>[2x]MCF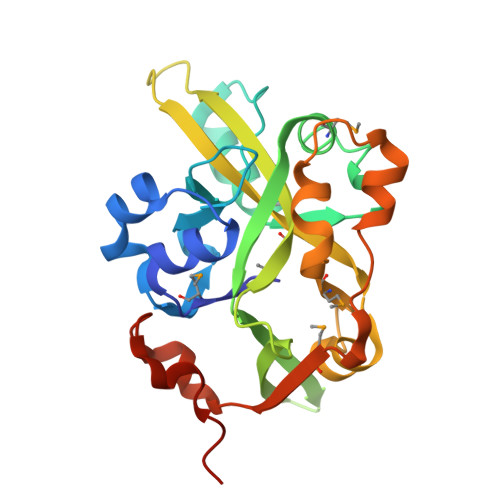HNSMSAKAIKVAARYGRQSDVVEIYQSILDEQYHVNAFTFPRYPIITSSDEVQVFNWGLIPFWVRSEEDATEIRKMTLNARADTIFEKPSFREPIMKKRCIVPSTGYFEWRHEGANKIPYYIYVKDEPIFSMAGIYDRWLDKDTGEEHETFSIITTDTNSLTDYIDNTKHRMPAILTQEEEEKWLNPSLSKAEIASLLKPFDTEKMDAYVIRNDFLKKSPNDPTIVQRALEHHHHHH(R)-{1-[(2,5-dimethylphenyl)methyl]-6-(1-methyl-1H-pyrazol-4-yl)-1H-benzimidazol-2-yl}(pyridin-4-yl)methanol 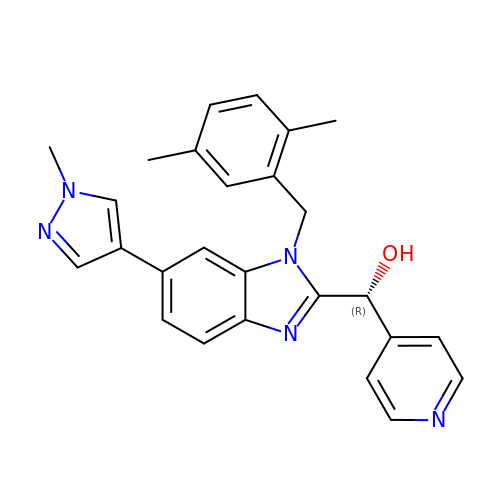| C26 H25 N5 O | RZGFWGNCSYUEPR-RUZDIDTESA-N> ENSEVIKDLYEYLCNVRVHKSYEDDSGLWFDISQGTHSGGSSDDYSIMDYKLGFVKGQAQVTEVIYAPVLKQRSTEELYSLQSKLPEYLFETLSFPLSSLNQFYNKIAKSLNKKREKKDETE;> AEF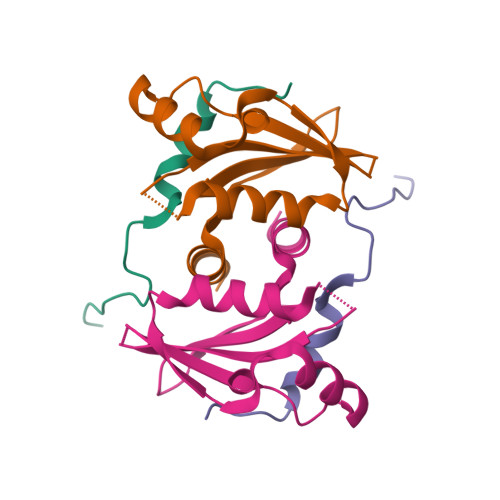TSPYFGRPSLKTRAKQFEGVSSP> MVEKEEAGGGISEEEAAQYDRQIRLWGLEAQKRLRASRVLLVGLKGLGAEIAKNLILAGVKGLTMLDHEQVTPEDPGAQFLIRTGSVGRNRAEASLERAQNLNPMVDVKVDTEDIEKKPESFFTQFDAVCLTCCSRDVIVKVDQICHKNSIKFFTGDVFGYHGYTFANLGEHEFVEEKTKVAKVSQGVEDGPDTKRAKLDSSETTMVKKKVVFCPVKEALEVDWSSEKAKAALKRTTSDYFLLQVLLKFRTDKGRDPSSDTYEEDSELLLQIRNDVLDSLGISPDLL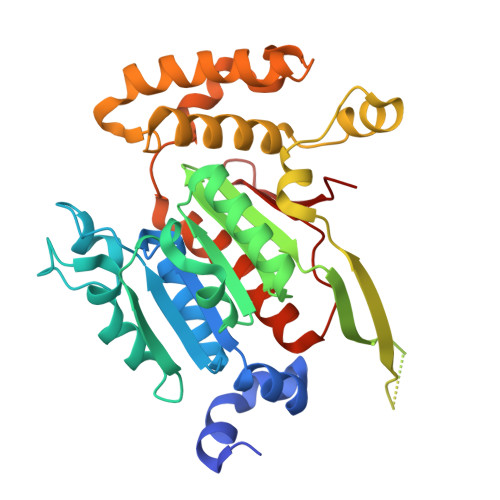PEDFVRYCFSEMAPVCAVVGGILAQEIVKALSQRDPPHNNFFFFDGMKGNGIVECLGPK> MSLALSQIEIQQFLSEAHAEFQSEGFLLQGAVRTKSGTKGSIVHFPVFGEGMANQKAPQDDITPMNVSNRDAEAVIEDWYASEYADRSFQNKLAVNAVEEYAKLCAWAIGRRADQINIDTIAGATYSATPNDQQGALVPVGTTGFTFEKLRQAHRWLRQRSANRGKRTVIIDAIAEE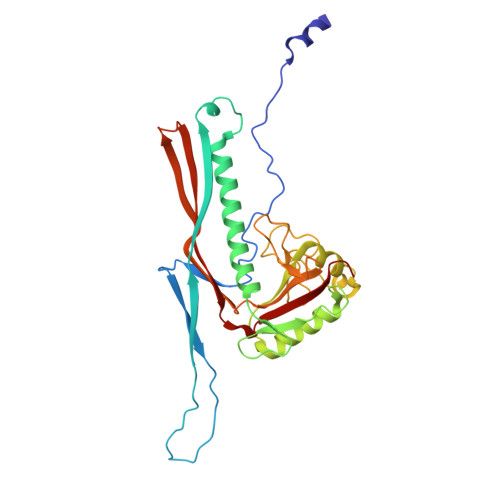QLLNVEQLTNSFYVNQKILDNDGLHGMTFLGMNFIVIPSMQEGGLPTTGGGTVGRAFFINEMAVGYAQSERLGGDISWENIKTSYLINMWMEAGAVVIDPKGLVEVDYLLEP>[2x]NEGKALMAIKASFSNVANMLLDWDDVHNHDFCSWRGVFCDNVSLNVVSLNLSNLNLGGEISSALGDLMNLQSIDLQGNKLGGQIPDEIGNCVSLAYVDFSTNLLFGDIPFSISKLKQLEFLNLKNNQLTGPIPATLTQIPNLKTLDLARNQLTGEIPRLLYWNEVLQYLGLRGNMLTGTLSPDMCQLTGLWYFDVRGNNLTGTIPESIGNCTSFEILDVSYNQITGVIPYNIGFLQVATLSLQGNKLTGRIPEVIGLMQALAVLDLSDNELTGPIPPILGNLSFTGKLYLHGNKLTGQIPPELGNMSRLS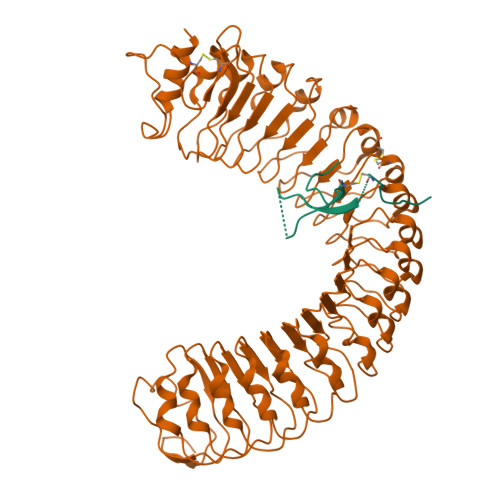YLQLNDNELVGKIPPELGKLEQLFELNLANNNLVGLIPSNISSCAALNQFNVHGNFLSGAVPLEFRNLGSLTYLNLSSNSFKGKIPAELGHIINLDTLDLSGNNFSGSIPLTLGDLEHLLILNLSRNHLNGTLPAEFGNLRSIQIIDVSFNFLAGVIPTELGQLQNINSLILNNNKIHGKIPDQLTNCFSLANLNISFNNLSGIIPPMKNFTRFSPASFFGNPFLCGNWVGSICGPHHHHHH;>PGSSPPTCRSKCGKCQPCKPVHVPIQPGLSMPLEYYPEAWRCKCGNKLFMP[2x]> MSTVKAPTLPASIFRAYDIRGVVGDTLTAETAYWIGRAIGSESLARGEPCVAVGRDGRLSGPELVKQLIQGLVDCGCQVSDVGMVPTPVLYYAANVLEGKSGVMLTGSHNPPDYNGFKIVVAGETLANEQIQALRERIEKNDLASGVGSVEQVDILPRYFKQIRDDIAMAKPMKVVVDCGNGVAGVIAPQLIEALGCSVIPLYCEVDGNFPNHHPDPGKPENLKDLIAKVKAENADLGLAFDGDGDRVGVVTNTGTIIYPDRLLMLFAKDVVSRNPGADIIFDVKCTRRLIALISGYGGRPVMWKTGHSLIKKKMKETGALLAGEMSGAVFFKERWFGFDDGIYSAARLLEILSQDQRDSEHVFSAFPSDISTPEINITVTEDSKFAIIEALQRDAQWGEGNITTLDGVRVDYPKGWG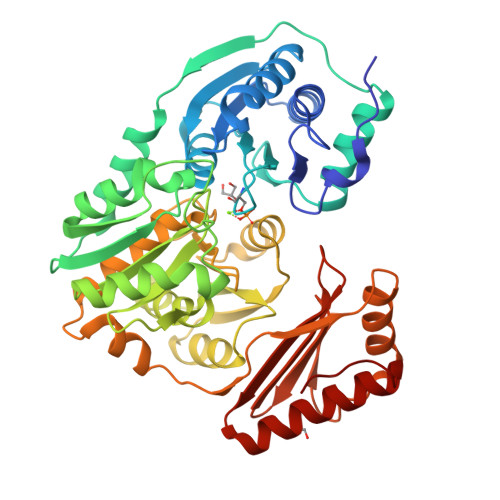LVRASNTTPVLVLRFEADTEEELERIKTVFRNQLKAVDSSLPVPF>MSLSELSPCHVRSGRIMTVDGPIPSSALGHTLMHEHLQNDCRCWWNPPQEPERQYLAEAPISIEILSELRQDPFVNKHNIALDDLDLAIAEVKQFAAVGGRSIVDPTCRGIGRDPVKLRRISAETGVQVVMGAGYYLASSMPETAARLSADDIADEIVAEALEGTDGTDARIGLIGEIGVSS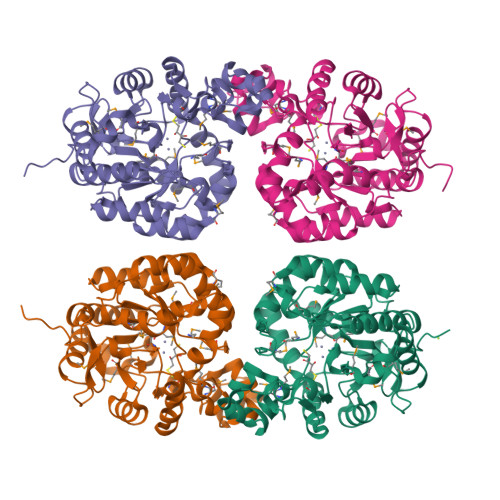DFTAEEEKSLRGAARAQVRTGLPLMVHLPGWFRLAHRVLDLVEEEGADLRHTVLCHMNPSHMDPVYQATLAQRGAFLEFDMIGMDFFYADQGVQCPSDDEVARAILGLADHGYLDRILLSHDVFVKMMLTRYGGNGYAFVTKHFLPRLRRHGLDDAALETLMVTNPRRVFDASIEGHHHHHH[4x]> GAMGSKNWFKITIPYGRKYDKAWLLSMIQSKCSVPFTPIEFHYENTRAQFFVEDASTASALKAVNYKILDRENRRISIIINSSAPPHTILNELKPEQVEQLKLIMSKRYDGSQQALDLKGLRSDPDLVAQNIDVVLNRRSCMAATLRIIEENIPELLSLNLSNNRLYRLDDMSSIVQKAPNLKILNLSGNELKSERELDKIKGLKLEELWLDGNSLCDTFRDQSTYISAIRERFPKLLRLDGHELPPPIAFDVEAPTTLPPCKGSYF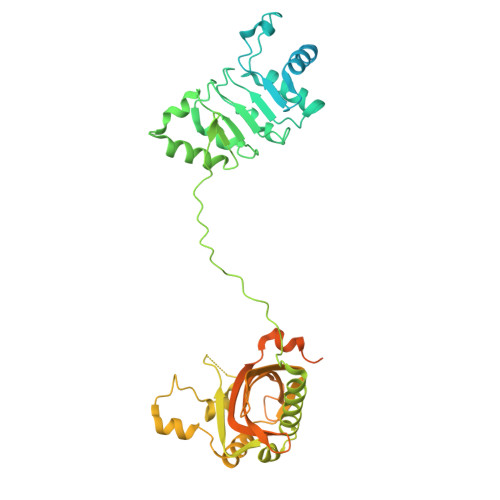GTENLKSLVLHFLQQYYAIYDSGDRQGLLDAYHDGACCSLSIPFIPQNPARSSLAEYFKDSRNVKKLKDPTLRFRLLKHTRLNVVAFLNELPKTQHDVNSFVVDISAQTSTLLCFSVNGVFKEVDGKSRDSLRAFTRTFIAVPASNSGLCIVNDELFVRNASSEEIQRAFAMPAPTPSSSPVPTLSPEQQEMLQAFSTQSGMNLEWSQKCLQDNNWDYTRSAQAFTHLKAKGEIPEVAFMK>[12x]QSPAEIASFSPRPSLADSKAVLN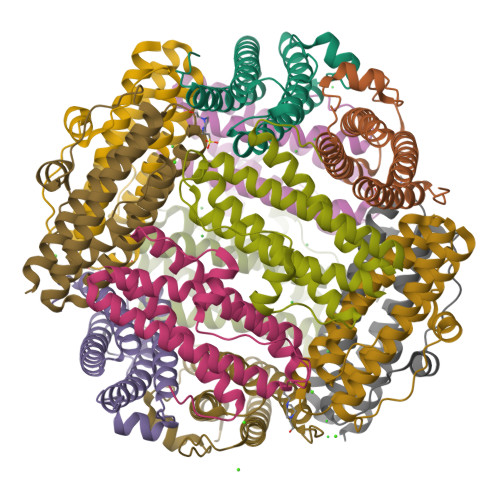QAVADLSVAHSILHQVHWYMRGRGFMIWHPKMDEYMEEIDGYLDEMSERLITLGGAPFSTLKEFSENSQLKEVLGDYNVTIEEQLARVVEVFRYLAALFQKGFDVSDEEGDSVTNDIFNVAKASIEKHIWMLQAELGQAPKL Afamin is a human plasma glycoprotein and a member of the albumin gene family that has been reported to be a multifunctional transporter of hydrophobic molecules such as vitamin E and a potential binding partner for Wnt signalling proteins. The structural similarity of afamin to hSA suggests that afamin might also be able to transport cargo in the bloodstream. The availability of four independent afamin structure models from two different crystal forms provides insight into the flexibility and dynamics of the molecule, which point towards a significant conformational adaptability when binding to hydrophobic molecules, metal chelates or proteins with hydrophobic acylation such as Wnt, supporting the potential function of afamin as a promiscuous transport molecule in human plasma.

Tissue-specific transport by afamin could greatly enhance the resolution of MRI imaging in blood-flow studies. As no crystal structure of albumin with a contrast agent is yet available, we selected gadoteridol (Gd-DO3A), which is used in medical applications as an MRI contrast agent and in crystallography as a lanthanide phasing compound. We were able to identify likely Gd-binding sites in a similar orthorhombic, low-resolution electron-density map of afamin by co-crystallization with Gd-DO3A. An even more dramatic cell contraction dominated by a further 6 Å contraction in a compared with the isomorphous ortho­rhombic dehydrated crystals and an almost 13% decrease from the monoclinic cell volume occurs in the orthorhombic afamin–Gd-DO3A complex crystals. Whether this decrease in cell volume is mediated by the single Gd-DO3A molecule located at a crystal contact or is a result of shifting local charge distributions owing to the lower crystallization pH of 5.5 versus 6.5 for native afamin remains unknown. After a few rounds of rebuilding it became clear that large parts of the protein had become severely disordered in the Gd-DO3A co-crystals, and owing to streaking and discontinuity in many parts of the map the model could not be completed. Subsequent occupancy refinement indicated Gd occupancies of between 0.9 and 0.7. The protrusions in the large density blobs and difference density suggested additional features around the Gd atom, but we were unable to determine and refine the orientation of the DO3A ‘crown’ around the Gd-DO3A. Our proposition of Gd-DO3A being present in afamin is based on a preponderance of evidence in the form of plausibility arguments, augmenting the reasonable evidence for strong Gd difference density. The validation report for the Gd model states an automatically extracted resolution limit of 2.69 Å.

> LPTQPRDIENFNSTQKFIEDNIEYITIIAFAQYVQEATFEEMEKLVKDMVEYKDRCMADKTLPECSKLPNNVLQEKICAMEGLPQKHNFSHCCSKVDAQRRLCFFYNKKSDVGFLPPFPTLDPEEKCQAYESNRESLLNHFLYEVARRNPFVFAPTLLTVAVHFEEVAKSCCEEQNKVNCLQTRAIPVTQYLKAFSSYQKHVCGALLKFGTKVVHFIYIAILSQKFPKIEFKELISLVEDVSSNYDGCCEGDVVQCIRDTSKVMNHICSKQDSISSKIKECCEKKIPERGQCIINSNKDDRPKDLSLREGKFTDSENVCQERDADPDTFFAKFTFEYSRRHPDLSIPELLRIVQIYKDLLRNCCNTENPPGCYRYAEDKFNETTEKSLKMVQQECKHFQNLGKDGLKYHYLIRLTKIAPQLSTEELVSLGEKMVTAFTTCCTLSEEFACVDNLADLVFGELCGVNENRTINPAVDHCCKTNFAFRRPCFESLKADKTYVPPPFSQDLFTFHADMCQSQNEELQRKTDRFLVNLVKLKHELTDEELQSLFTNFANVVDKCCKAESPEVCFNEESPKIGNKGENLYFQ>MTGTVSRRKKIAMIGSGMIGGTMGYLCVLRELADVVLFDVVTGMPEGKALDDSQATSIADTNVSVTSANQYEKIAGSDVVIITAGLTKVPGKSDKEWSRNDLLPFNAKIIREVAQGVKKYCPLAFVIVVTNPLDCMVKCFHEASGLPKNMVCGMANVLDSARFRRFIADQLEISPRDIQATVIGTHGDHMLPLARYVTVNGFPLREFIKKGKMTEAKLAEIVERTKKAGGEIVRLLGQGSAYYAPALSAITMAQAFLKDEKRVLPCSVYCQGEYGLHD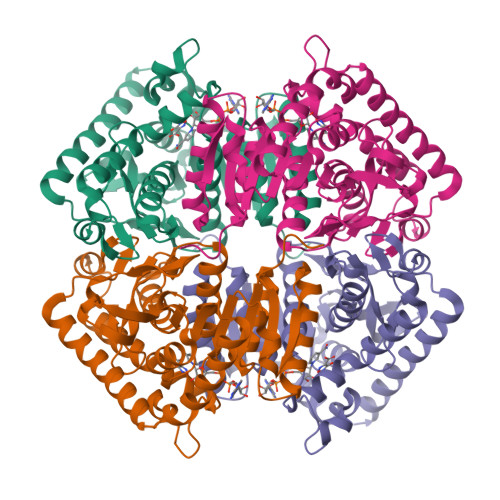MFIGLPAVIGGGGIEQVIELELTHEEQECFRKSVDDVVELNKSLAALG[2x]> AQSVPYGVSQIKAPALHSQGYTGSNVKVAVIDSGIDSSHPDLKVAGGASMVPSETNPFQDNNSHGTHVAGTVAALNNSIGVLGVAPSASLYAVKVLGADGSGQYSWIINGIEWAIANNMDVINMSLGGPS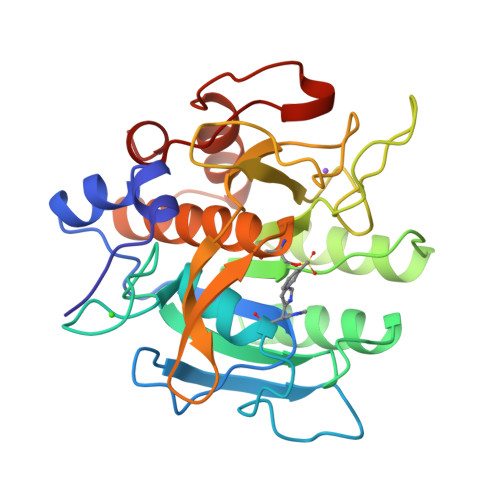GSAALKAAVDKAVASGVVVVAAAGNEGTSGSSSTVGYPGKYPSVIAVGAVDSSNQRASFSSVGPELDVMAPGVSIQSTLPGNKYGAYNGTSMASPHVAGAAALILSKHPNWTNTQVRSSLENTTTKLGDSFYYGKGLINVQAAAQ>GMRLPLNQRVAILLHEGTTGTIGKTGLALLRYSEAPIVAVIDRNCAGQSLREITGIYRYVPIVKSVEAALEYKPQVLVIGIAPKGGGIPDDYWIELKTALQAGMSLVNGLHTPLANIP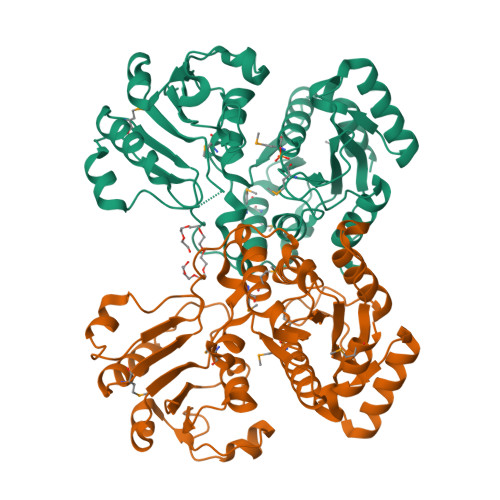DLNALLQPGQLIWDVRKEPANLDVASGAARTLPCRRVLTVGTDMAIGKMSTSLELHWAAKLRGWRSKFLATGQTGVMLEGDGVALDAVRVDFAAGAVEQMVMRYGKNYDILHIEGQGSLLHPGSTATLPLIRGSQPTQLVLVHRAGQTHNGNNPHVPIPPLPEVIRLYETVASGGGAFGTVPVVGIALNTAHLDEYAAKEAIAHTIAETGLPCTDVVRFGADVLLDAVMQN[4x]> IVGGTASVRGEWPWQVTLHTTSPTQRHLCGGSIIGNQWILTAAHCFYGVESPKILRVYSGILNQSEIKEDTSFFGVQEIIIHDQYKMAESGYDIALLKLETTVNYTDSQRPISLPSKGDRNVIYTDCWVTGWGYRKLRDKIQNTLQKAKIPLVTNEECQKRYRGHKITHKMICAGYREGGKDACKGDSGGPLSCKHNEVWHLVGITSWGEGCAQRERPGVYTNVVEYVDWILEKTQAV

Activated coagulation factor XI (FXIa) is a highly attractive antithrombotic target as it contributes to the development and progression of thrombosis but is thought to play only a minor role in hemostasis so that its inhibition may allow for decoupling of antithrombotic efficacy and bleeding time prolongation. Recently, another serine protease in the coagulation cascade, factor XIa (FXIa),7 has emerged as an attractive target, because it may allow for a more selective reduction of fibrin generation: FXI is activated via FXIIa after contact activation or by thrombin in the course of the positive feedback loop for thrombin amplification, but it is not involved in the tissue factor pathway, which is key for fibrin production to cover a vessel wall leakage. Thus, this form of “selective coagulation modulation”8 by FXIa inhibition may allow for a decoupling of antithrombotic efficacy and bleeding risk and offer the opportunity for better antithrombotic protection to a much broader patient population. In this study, we describe our drug discovery efforts, resulting in the identification of asundexian (BAY 2433334, 80), a direct, potent, selective, and reversible small molecule FXIa inhibitor for oral application, which is currently being investigated in clinical Phase 3 trials.

To explore FXIa inhibitors, we synthesized tetrazole 1 (inspired by chemical matter published by Bristol Myers Squibb in 200723) which showed good potency (FXIa IC50 = 9 nM). A docking experiment of this compound in the published X-ray structure of FXIa24 indicated that the 4-aminomethyl-trans-cyclohexyl residue would occupy the S1 pocket. An X-ray cocrystal structure of tetrazole 1 in complex with human FXIa then revealed the binding mode with the key hydrogen bonds and hydrophobic contacts. The 4-aminomethyl-trans-cyclohexyl moiety was indeed found to be located in the S1 pocket where its primary amine forms a direct ionic interaction with the carboxylate of Asp189 and a hydrogen bond with the backbone carbonyl of Gly218. The S1 pocket is the only deep pocket of the FXIa active site, and ligand 1 extends from the S1 pocket into the S1′ and S2′ pockets. We hypothesized that this orientation in the binding mode toward the prime sites might facilitate the required selectivity versus other serine proteases such as FXa and thrombin, as potent inhibitors of the latter use the more druggable pockets of their nonprime site (S1 and S2; S4).25 The cyclohexyl-bound amide carbonyl oxygen forms two hydrogen bonds with the protein backbone forming the oxyanion hole (OAH in Figure 1). The ester binding pocket (EBP) is not occupied with substituents of 1. Located in the S2′ pocket, the tetrazole moiety of 1 forms a hydrogen bond with the hydroxyl group of Tyr143 and a water-mediated interaction with the carbonyl group of His38. In the S1′ pocket, the phenyl ring of the benzyl side chain participates in a hydrophobic contact with the Cys42-Cys58 disulfide bridge.>ESGKASSSLGLQDFDLLRVIGRGSYAKVLLVRLKKTDRIYAMKVVKKELVNDDEDIDWVQTEKHVFEQASNHPFLVGLHSCFQTESRLFFVIEYVNGGDLMFHMQRQRKLPEEHARFYSAEISLALNYLHERGIIYRDLKLDNVLLDSEGHIKLTDYGMCKEGLRPGDTTSTFCGTPNYIAPEILRGEDYGFSVDWWALGVLMFEMMAGRSPFDIVGSSDNPDQNTEDYLFQVILEKQIRIPRSLSVKAASVLKSFLNKDPKERLGCHPQTGFADIQGHPFFRNVDWDMMEQKQVVPPFK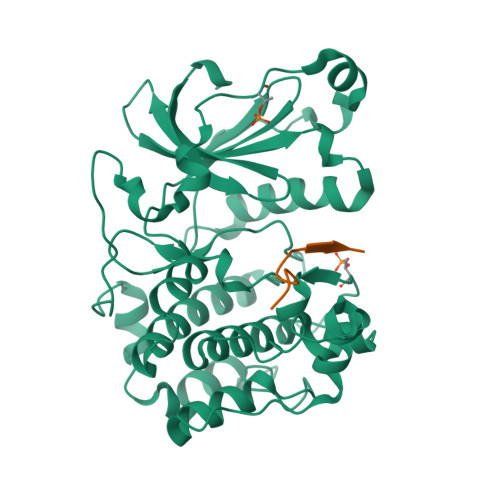PNISGEFGLDNFDSQFTNEPVQLTPDDDDIVRKIDQSEFEGFEYINPLLMSAEECV[2x];>[2x]SRVKSLKKSLRQSFRRMRKS2,3-DIHYDROXYBENZALDEHYDE 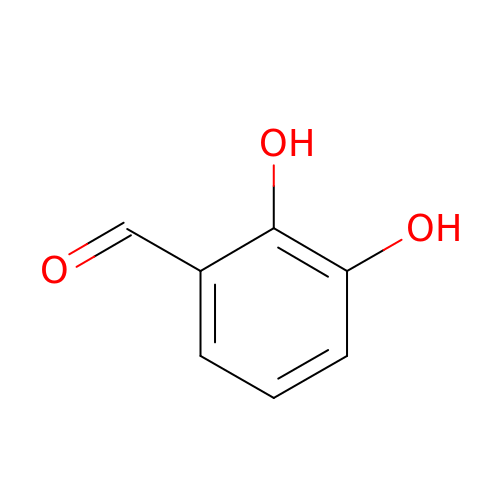| C7 H6 O3 | IXWOUPGDGMCKGT-UHFFFAOYSA-N1,2-dimethylquinolin-4-imine | C11 H12 N2 | 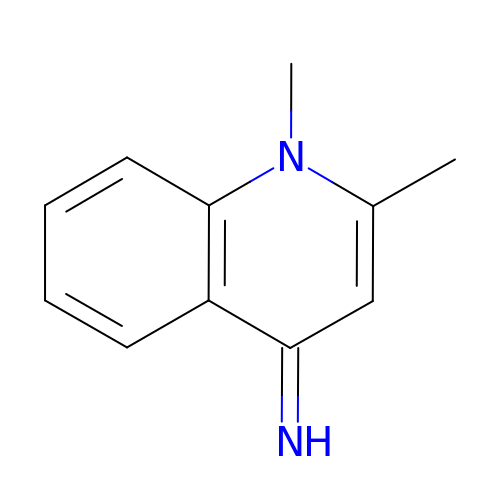LUHYAOUKGPHLIP-ZRDIBKRKSA-N>KVLKISQTKYEEILKISKKYIFINQVDKSFHEAVDDLNQQDFIAVSGDGANMGRKCKMPFLVLSTDHQIYIFDIQVMQYHAFESGLKKILEGDSPKKIAHDCRKLSDCLYHKHNVKLKSVFDTQVGDLIITKNKKVTLPNKVKSLGECLTNYLGLQQNTIDEKLDIVQSTERPLSVKIKDSLARNIAFLHHLSEVINEEMQLPFYRGVECYIENIRSSDDFKAWELCGKLNQIPKEF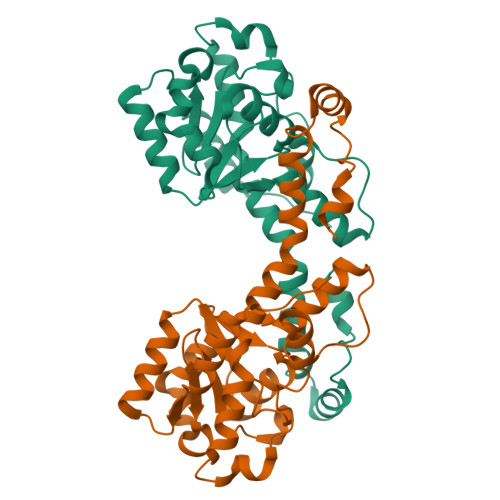RNAIDY[5x]>AYSTREILLALCIRDSRVHGNGTLHPVLELAARETPLRLSPEDTVVLRYHVLLEEIIERNSETFTETWNRFITHTEHVDLDFNSVFLEIFHRGDPSLGRALAWMAWCMHACRTLCCNQSTPYYVVDLSVRGMLEASEGLDGWIHQQGGWSTLIEDN[5x];>[5x]DIIRNIARHL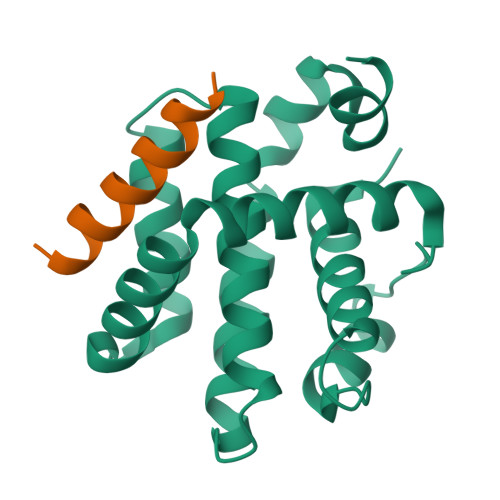AQVGDSMD> MAHCTEYMNAPKKLPADVAEELATTAQKLVQAGKGILAADESTQTIKKRFDNIKLENTIENRASYRDLLFGTKGLGKFISGAILFEETLFQKNEAGVPMVNLLHNENIIPGIKVDKGLVNIPCTDEEKSTQGLDGLAERCKEYYKAGARFAKWRTVLVIDTAKGKPTDLSIHETAWGLARYASICQQNRLVPIVEPEILADGPHSIEVCAVVTQKVLSCVFKALQENGVLLEGALLKPNMVTAGYECTAKTTTQDVGFLTVRTLRRTVPPALPGVVFLSGGQSEEEASVNLNSINALGPHPWA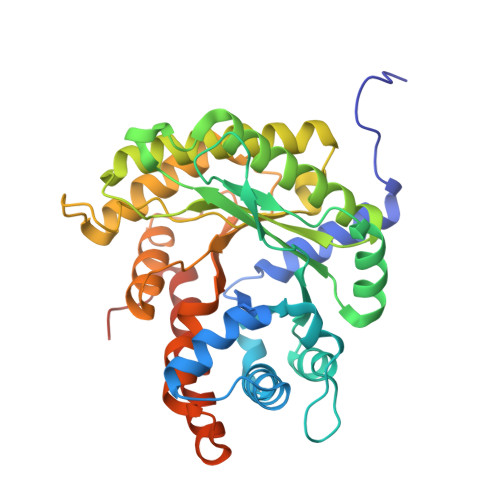LTFSYGRALQASVLNTWQGKKENVAKAREVLLQRAEANSLATYGKYKGGAGGENAGASLYEKKYVY>MYDNSISGLTEEQAKEFHEQFKTTFTVFMVLAAAAHFLVFLWRPFY[8x];>MSEYRPSKPSNPRDDWKLWLVVNPGTWLMPILMAVLVVALVVHAFVYSNDNYNPLTFDASAEVA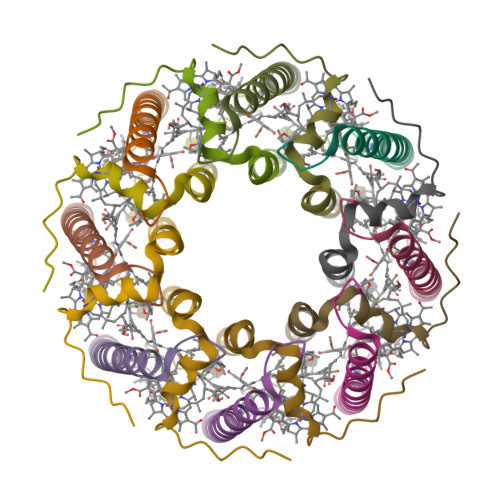AEEAAE[8x]> MVSVNENALPLVERMIERAELLNVEVQELENGTTVIDCGVEAAGGFEAGLLFSEVCMGGLATVELTEF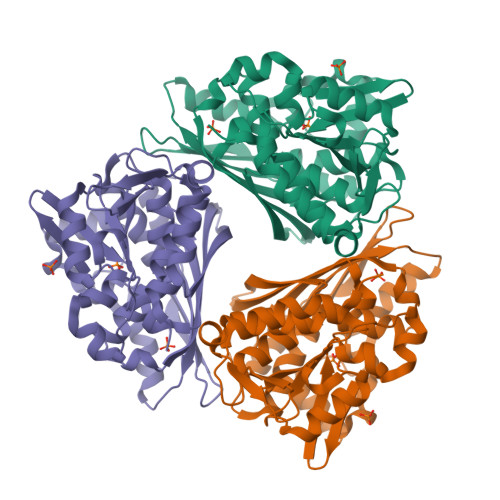EHDGLCLPAVQVTTDHPAVSTLAAQKAGWQVQVGDYFAMGSGPARALALKPKETYEEIDYEDDADVAILCLESSELPDEDVAEHVADECGVDPENLYLLVAPTASIVGSVQVSARVVETGLYKLLEVLEYDVTRVKYATGTAPIAPVADDDGEAMGRTNDCILYGGTVYLYVEGDDELPEVVEELPSEASEDYGKPFMKIFEEADYDFYKIDPGVFAPARVVVNDLSTGKTYTAGEINVDVLKESFSL> SMNNSIKFHVSYDGTARALFNTKEQAEKYCLVEEINDEMNGYKR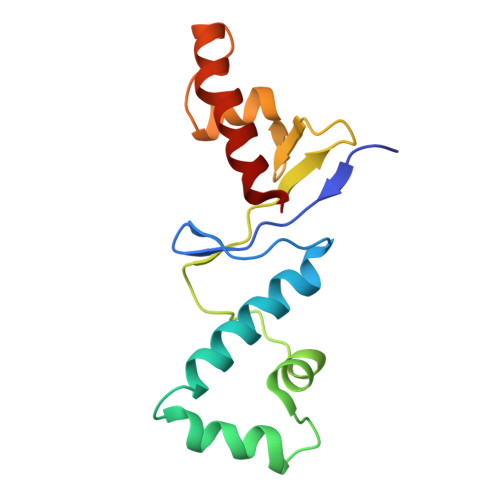KSWEEKLREENCASVQDWVEKNYTSSYSDLFNICEIEVSSAGQLVKIDNTEVDDFVENCYGFTLEDDLEEFNKAKQYLQKFYAECEN> MRVFHRLSTAHDDLIHDVSYDFYGKRLATCSSDQKIKVWDQNDNQKWELSAEWKAHSGSVWKLAWAHPEYGQVIASCSFDRTVCIWEESEDEKGQKKWQLKAHLVDSRDSVTDIKFAPKSFGLRLATCSSDGYIRIYEAMDIMNLSQWTIVEEFESQKGTSNCISWNPSSYDKPMIAVGSNEPYIKIWEYSETARKWLQIDTLTAYPIGSTISSSNLNSGGGIGGGIGSGIGGGIGGGIGGAGGSIGGVSGVNNSSMGNLGSGIGNNINN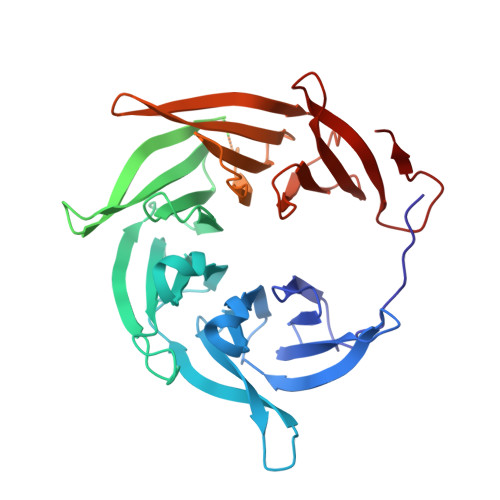SNINNISVGVGSGVGGGVGSGVGGSLNNGLNSAQGNSIGNGNIGSLNNISGNSGGLNSNSLMSGANSSINVSSGNNSIYSNNNFDSSSDGGSRAIHDVCWAPNMGRSYHLIATASKDHKVRIWKLSSDKSKMELKEVMRKDDHKSEVWRVEWNITGTILASSGDDGNVCLWKCNMNGEWKLFSLISGEESTEDKYDR>SEELEKALSKLSEREAMVLKMRKGLIDGREHTLEEVGAYFGVTRERIRQIENKALRKLRHPSRSEKLRDFLE[2x];>K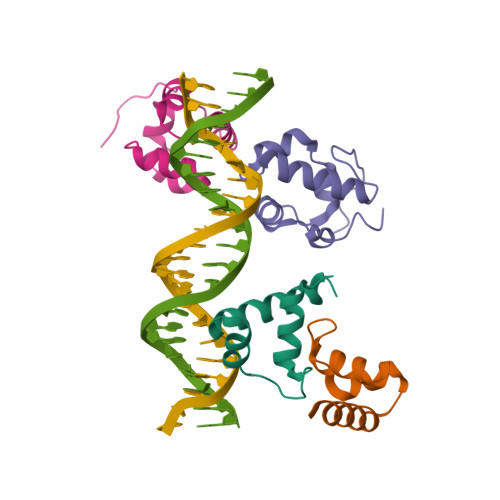PEFDPILLRPVDDLELTVRSANCLKAEAIHYIGDLVQRTEVELLKTPNLGKKSLTEIKDVLASRGLSLGMRLENWPPASIADE[2x]> GSHMINVNKKALGQDTEKMEEQLDLLSAILDPSKS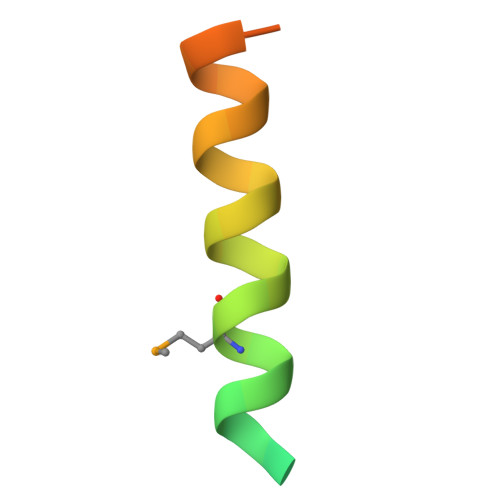KGAGS>GPLGSMYHLPDM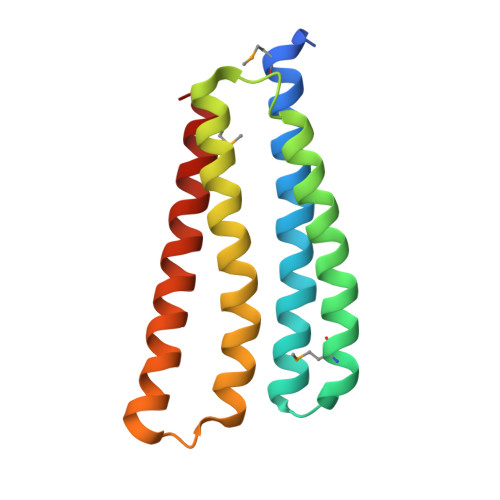EETVNKILRAQETRAQLYKELEDALNANQEKKIGLEQMGIIVQLVTEGLNEVSSDIRNYQASLTKELKLLVDSLQEKERSKLQATVKLEQLKVVSTNSPVENTQISELEARLSSLSKEINDILQNMKDEI[8x]> MKELIYIEEPKILFAHGQKCTDARDGLALFGPLNNLYGIKSGVIGTKQGLKIF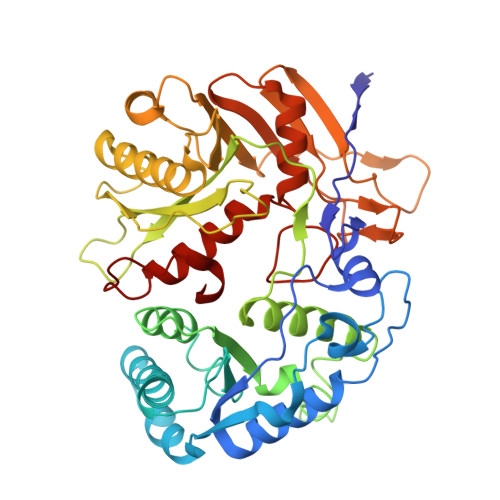RDYLDHIQKPIYNSNSITRPMFPGFEAVFDCKWESTGITFKEVTNEDIGKFLYNSSTHKRTYDLVSLFIDKIISANKNEDENVDVWFVIVPDEIYKYCRPNSVLPKEMVQTKALMSKSKAKSFRYEPSLFPDINIELKEQEKEAETYNYDAQFHDQFKARLLKHTIPTQIFRESTLAWRDFKNAFGLPIRDFSKIEGHLAWTISTAAFYKAGGKPWKLSDVRNGVCYLGLVYKKVEKSKNPRNACCAAQMFLDNGDGTVFKGEVGPWYNPKNGQYHLEPKEAKALLSQSLQSYKEQIGEYPKEVFIHAKTRFNHQEWDAFLEVTPKETNLVGVTISKTKPLKLYKTEGDYTILRGNAYVVNERSAFLWTVGYVPKIQTALSMEVPNPLFIEINKGEADIKQVLKDILSLTKLNYNACIFADGEPVTLRFADKIGEILTASTDIKTPPLAFKYY>ISKKQDEGVVVNKFRPKEPYIGRCLL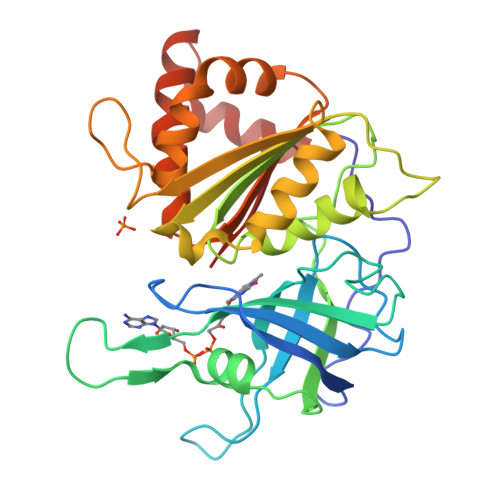NTKITGDDAPGETWHMVFSTEGEIPYREGQSIGVIADGVDANGKPHKLRLYSIASSALGDFGDSKTVSLCVKRLVYTNDKGEEVKGVCSNFLCDLKPGADVKITGPVGKEMLMPKDPNATVIMLGTGTGIAPFRSFLWKMFFEKHDDYKFNGLAWLFLGVPTSSSLLYKEEFEKMKEKAPENFRLDFAVSREQTNEKGEKMYIQTRMAQYAEELWTLLKKDNTFVYMCGLKGMEQGIDDIMSSLAAKEGIDWADYKKQLKKAEQWNVEVY[2x]> MSAIKPDMKIKLRMEGNVNGHHFVIDGDGTGKPFEGKQSMDLEVKEGGPLPFAFDILTTAFAYGNRVFAKYPDNIQDYFKQSFPKGYSWERSLTFEDGGICNARNDITMEGDTFYNKVRFYGTNFPANGPVMQKKTLKWEPSTEKMYVRDGVLTGDVETALLLEGNAHYRCDFRTTYKAKEKGVKLPGAHFVDHCIEILSHDKDYNKVKLYEHAVAHSGLPN

Based on the EosFP sequence, we developed a new reversibly photoswitching rs-FP, ‘rsKiiro’ (described in detail in Supplementary Discussion 10). Reversible photoswitching occurs between a bright fluorescent cis anionic p-hydroxybenzylideneimidazolinone (HBDI) chromophore (the ‘on’ state) and the non-fluorescent trans neutral (the ‘off’ state), as is also the case for the rs-FP ‘Dronpa’. Compared to Dronpa, rsKiiro has substantially improved structural ordering in the ‘on’ ground state as well as the ‘off’ photoproduct, allowing high-resolution X-ray crystallography of the photoreactions. Illumination of the ‘on’ state with green light drives a cis–trans photoisomerization of the chromophore to produce a metastable non-fluorescent ‘off’ state with a neutral trans chromophore.

An ~100-fs pump interaction at 400 nm, close to resonance of the trans neutral chromophore (off state), creates an excited-state population with a lifetime of τ = 50 ps in both solution and crystals. A power density of 1,400 GW cm−2 (full-width at half-maximum, FWHM) was chosen for PP experiments to maximize the photoisomerization yield, based on optical measurements in crystals of anionic cis product absorption. The pump–probe observations up to 1-ps delay showed strong Fo–Fo difference electron-density features, up to 8.5σ, on the chromophore and on a hydrogen-bonded water and throughout the core of the protein. Coordinate refinement from extrapolated structure factors and occupancy refinement showed a small translational motion of the chromophore characterized by a 69-pm displacement of the phenolic oxygen. A 1.25-Å coordinate change of a nearby hydrogen-bonded water molecule modifies the O–O distance between the chromophore and water from 2.63 Å to 3.06 Å. A concomitant repositioning of the Gly155 backbone carbonyl changes its O–O distance to this water molecule from 2.77 Å to 2.84 Å. The larger distances in the femtosecond time-resolved structure suggest that the hydrogen bonding of the water molecule to both the chromophore and Gly155 is weakened. Other water molecules in the chromophore pocket and the side chains that primarily reside on the central helix undergo similar rearrangements. However, the PDP data show stronger differences and a modified temporal dependence compared to the PP measurement after the Stokes ‘dump’ pulse was introduced, and there are no discernible signals that are depleted by stimulated emission pumping. This observation forms our primary motivation for assigning the structural changes observed in the PP conditions to dominating ground-state motion, which is unconnected to the photoisomerization reaction coordinate. The excited-state coherence is not impulsively prepared; it is purely displacement-driven and insufficiently ordered, whereas the cis anionic chromophore product state is seen after full electronic and population decay and thermal proton transfer.> MAESVTNPQRPPVIWIGAQECTGCTESLLRAT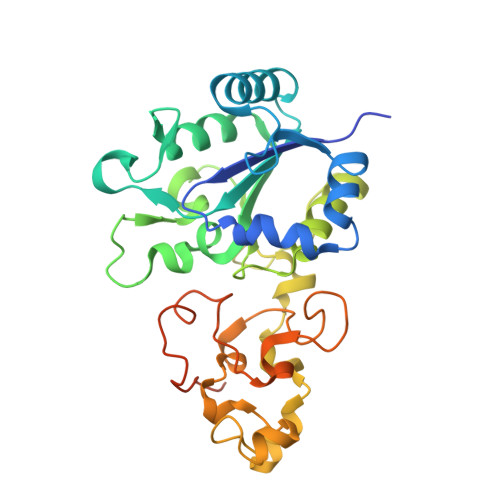HPTVENLVLETISLEYHEVLSAAFGHQVEENKHNALEKYKGQYVLVVDGSIPLKDNGIYCMVAGEPIVDHIRKAAEGAAAIIAIGSCSAWGGVAAAGVNPTGAVSLQEVLPGKTVINIPGCPPNPHNFLATVAHIITYGKPPKLDDKNRPTFAYGRLIHEHCERRPHFDAGRFAKEFGDEGHREGWCLYHLGCKGPETYGNCSTLQFCDVGGVWPVAIGHPCYGCNEEGIGFHKGIHQLANVENQTPRSQKPDVNAKEGGHHHHHH> FSEEEVRYEIILEKIRGTLKERPDEIAMLFKLLIKD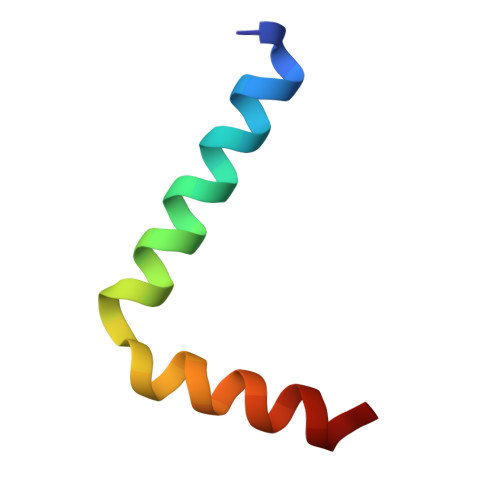E> MPPKKGGDGIKPPPIIGRFGTSLKIGIVGLPNVG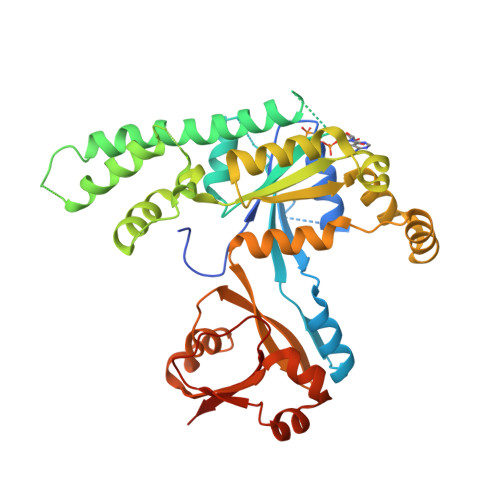KSTFFNVLTNSQASAENFPFCTIDPNESRVPVPDERFDFLCQYHKPASKIPAFLNVVDIAGLVKGAHNGQGLGNAFLSHISACDGIFHLTRAFEDDDITHVEGSVDPIRDIEIIHEELQLKDEEMIGPIIDKLEKVAVRGGDKKLKPEYDIMCKVKSWVIDQKKPVRFYHDWNDKEIEVLNKHLFLTSKPMVYLVNLSEKDYIRKKNKWLIKIKEWVDKYDPGALVIPFSGALELKLQELSAEERQKYLEANMTQSALPKIIKAGFAALQLEYFFTAGPDEVRAWTIRKGTKAPQAAGKIHTDFEKGFIMAEVMKYEDFKEEGSENAVKAAGKYRQQGRNYIVEDGDIIFFKFNTPQQPKKK>[2x]ETGRTEAAPAAGQPVESFPLDFTAVEGNMDSFMAQVKSLAQSLYPCSAQQLNEDLRLHLLLNTSVTCNDGSPAGYYLKESRGSRRWLLFLEGGWYCFNRENCDSRYDTMRRLMSSRDWPRTRTGTGILSSQPEENPYWWNANMVFIPYCSSDVWSGASSKSEKNEYAFMGALIIQEVVRELLGRGL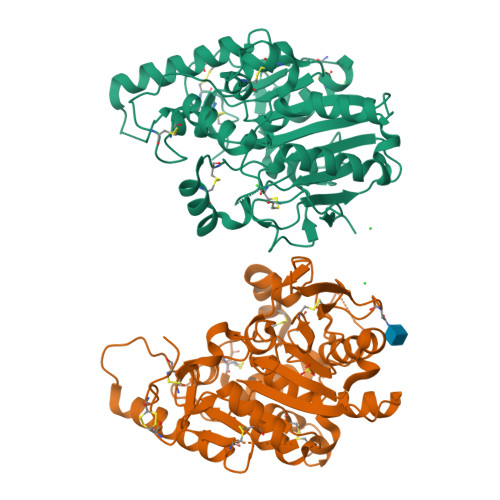SGAKVLLLAGSSAGGTGVLLNVDRVAEQLEKLGYPAIQVRGLADSGWFLDNKQYRHTDCVDTITCAPTEAIRRGIRYWNGVVPERCRRQFQEGEEWNCFFGYKVYPTLRCPVFVVQWLFDEAQLTVDNVHLTGQPVQEGLRLYIQNLGRELRHTLKDVPASFAPACLSHEIIIRSHWTDVQVKGTSLPRALHCWDRSLHDSHKASKTPLKGCPVHLVDSCPWPHCNPSCPTVRDQFTGQEMNVAQFLMHMGFDMQTVAQPQGLEPSELLGMLSNGSGTKHHHHHH>CG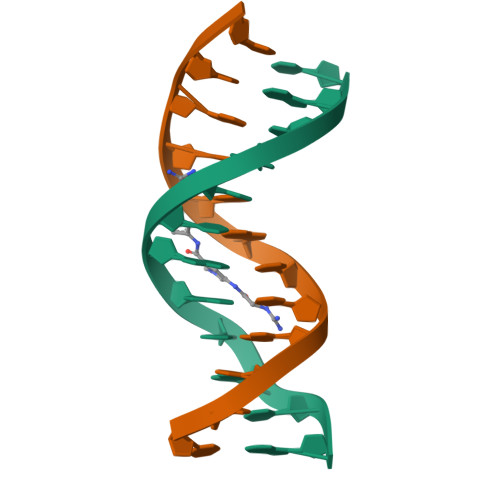CGTTAACGCG[2x]> GS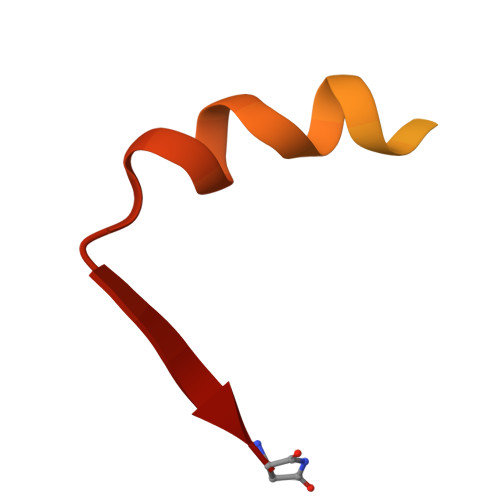HMASMSKDEVKREAKDTDGNPEIKGERRRLHSEIQSGSLANNIKKSTVIVKN>MGNLIKEDMRVKVHMEGNVNGHAFVIEGEGKGKPYEGTQTLNLTVKEGAPLPFSYDILTTALHYGNRVFTKYPEDIPDYFKQSFPEGYSWERTMTYEDKGICTIRSDISLEGDCFFQNVRFNGMNFPPNGPVMQKKTLKWEPSTEKLHVRDGLLVGNINMALLLEGGGHYLCD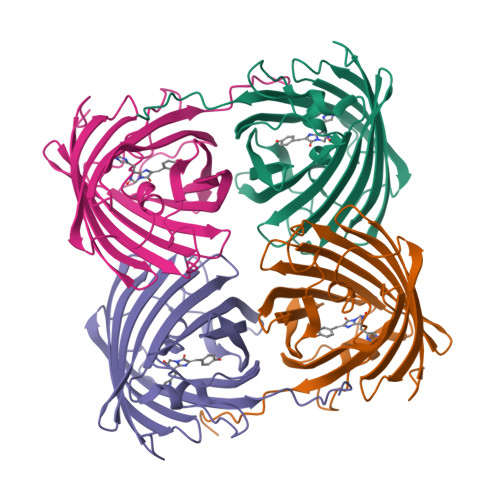FKTTYKAKKVVQLPDYHFVDHRIEILSNDSDYNKVKLYEHGVARYSPLPSQAWGSHHHHHH[16x]> 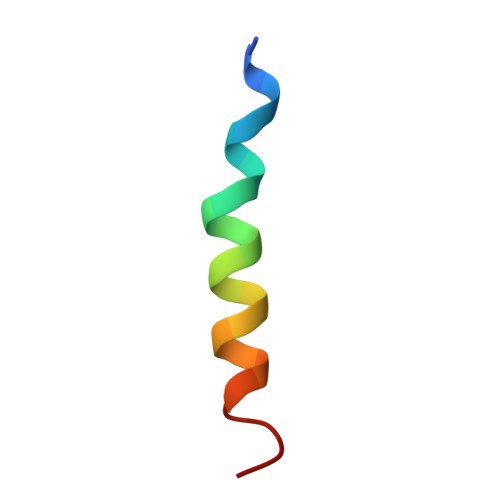NVTPFIDVMLVLLIIFMVAAPL3-(1,3,7-TRIHYDRO-9-D-RIBITYL-2,6,8-PURINETRIONE-7-YL) 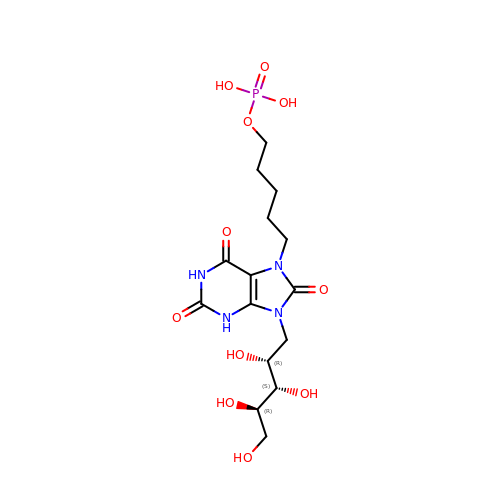1-PHOSPHATE | C15 H25 N4 O11 P | LVMWQWUPWMYMKX-KKZNHRDASA-N> NEGCAPLTGKESGMDIGRSSTERCLPGANPLQDQQWYLLNSGQDGFSARGGIAGNDLNLWWAHRTGVLGQGVNVAVVDDGLAIAHPDLADNVRPGSKNVVTGSDDPTPTDPDTAHGTSVSGIIAAVDNAIGTKGIAPRAQLQGFNLLDDNSQQLQKDWLYALGDSNASRDNRVFNQSYGMSVVDPRSANSLDQSQLDRLFEQQTLKAQGAAYIKAAGNGFNKIAAGGYVLNR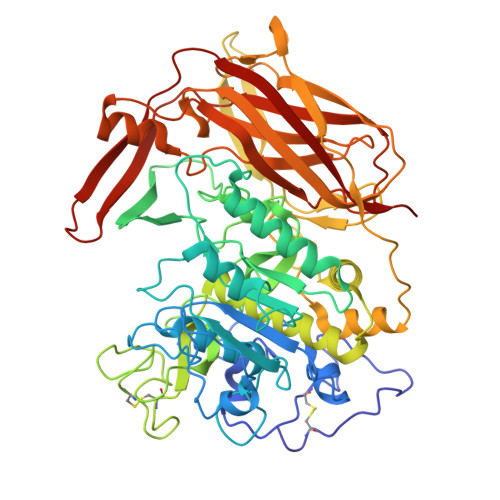TGNGPKLPFENSNLDPSNSNFWNLVVSALNADGVRSSYSSVGSNIFLSATGGEYGTDTPAMVTTDLPGCDMGYNRTDDPSTNRLHGNSQLDASCDYNGVMNGTASATPSTSGAMALLMSAYPDLSVRDLRDLLARSATRVDAKHQPVMVSYTSSTGKVRDVKGLEGWERNAAGMWFSPTYGFGLIDVNKALELAANHQPLPPLVQLPWQKINVTGSAAAIADVGNSPTSSTTRIATPLTVEAVQVMVSLDHQRLPDLLIELVSPAGTRSILLSPFNSLVGQSLDQQQLGFVRTKGLRDMRMLSNKFYGESAQGTWRLEVTDVANGTRQVSLLNRETRERTTLTERNNRQPGKLISWSLRVLGHDANRS>MSASRKTLVVTNDFPPRIGGIQSYLRDFIATQDPESIVVFASTQNAEEAHAYDKTLDYEVIRWPRSVMLPTPTTAHAMAEIIREREIDNVWFGAAAPLALMAGTAKQAGASKVIASTHGHEVGWSMLPGSRQSLRKIGTEVDVLTYISQYTLRRFKSAFGSHPTFEHLPSGVDVKRFTPATPEDKSATRKKLGFTDTTPVIACNSRLVPRKGQDSLIKAMPQVIAARPDAQLLIVGSGRYESTLRRLATDVSQNVKFLGRLEYQDMINTLAAADIFAMPARTRGGGLDVEGLGIVYLEAQACGVPVIAGTSGGAPETVTPATGLVVEGSDVDKLSELLIELLDDPIRRAAMGAAGRAHVEAEWSWEIMGERLTNILQSEPR[2x];>[2x]MGHHHHHHHHHHSSGHI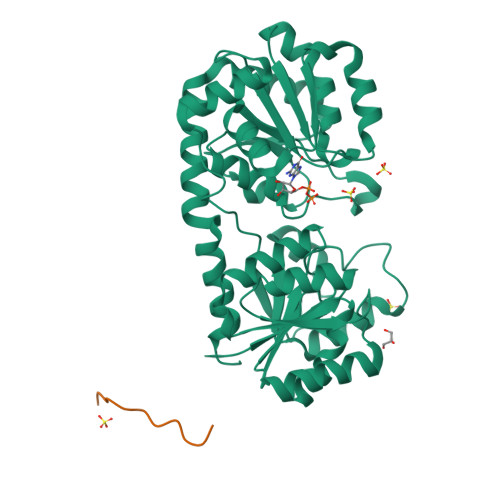EGRH> MAAFKPNSINYILGLDIGIASVGWAMVEIDEEENPIRLIDLGVRVFERAEVPKTGDSLAMARRLARSVRRLTRRRAHRLLRTRRLLKREGVLQAANFDENGLIKSLPNTPWQLRAAALDRKLTPLEWSAVLLHLIKHRGYLSQRKNEGETADKELGALLKGVAGNAHALQTGDFRTPAELALNKFEKESGHIRNQRSDYSHTFSRKDLQAELILLFEKQKEFGNPHVSGGLKEGIETLLMTQRPALSGDAVQKMLGHCTFEPAEPKAAKNTYTAERFIWLTKLNNLRILEQGSERPLTDTERATLMDEPYRKSKLTYAQARKLLGLEDTAFFKGLRYGKDNAEASTLMEMKAYHAISRALEKEGLKDKKSPLNLSPELQDEIGTAFSLFKTDEDITGRLKDRIQPEILEALLKHISFDKFVQISLKALRRIVPLMEQGKRYDEACAEIYGDHYGKKNTEEKIYLPPIPADEIRNPVVLRALSQARKVINGVVRRYGSPARIHIETAREVGKSFKDRKEIEKRQEENRKDREKAAAKFREYFPNFVGEPKSKDILKLRLYEQQHGKCLYSGKEINLGRLNEKGYVEIDHALPFSRTWDDSFNNKVLVLGSENQNKGNQTPYEYFNGKDNSREWQEFKARVETSRFPRSKKQRILLQKFDEDGFKERNLNDTRYVNRFLCQFVADRMRLTGKGKKRVFASNGQITNLLRGFWGLRKVRAENDRHHALDAVVVACSTVAMQQKITRFVRYKEMNAFDGKTIDKETGEVLHQKTHFPQPWEFFAQEVMIRVFGKPDGKPEFEEADTLEKLRTLLAEKLSSRPEAVHEYVTPLFVSRAPNRKMSGQGHMETVKSAKRLDEGVSVLRVPLTQLKLKDLEKMVNREREPKLYEALKARLEAHKDDPAKAFAEPFYKYDKAGNRTQQVKAVRVEQVQKTGVWVRNHNGIADNATMVRVDVFEKGDKYYLVPIYSWQVAKGILPDRAVVQGKDEEDWQLIDDSFNFKFSLHPNDLVEVITKKARMFGYFASCHRGTGNINIRIHDLDHKIGKNGILEGIGVKTALSFQ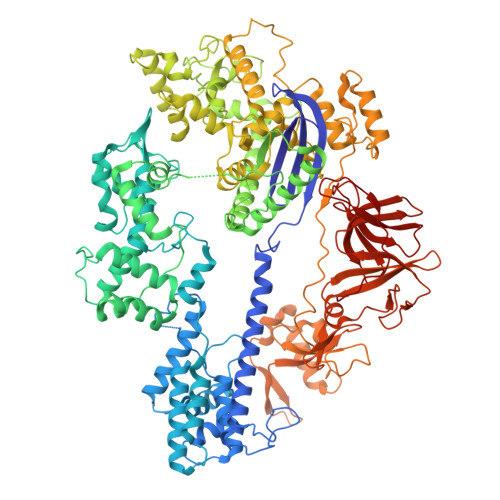KYQIDELGKEIRPCRLKKRPPVRSEHHHHHHHH> QGVNDNEEGFFSARGHRPLDKKREEAPSLRPAPPPISGGGYRARPAKAAATQKKVERKAPDAGGCLHADPDLGVLCPTGCQLQEALLQQERPIRNSVDELNNNVEAVSQTSSSSFQYMYLLKDLWQKRQKQVKDNENVVNEYSSELEKHQLYIDETVNSNIPTNLRVLRSILENLRSKIQKLESDVSAQMEYCRTPCTVSCNIPVVSGKECEEIIRKGGETSEMYLIQPDSSVKPYRVYCDMNTENGGWTVIQNRQDGSVDFGRKWDPYKQGFGNVATNTDGKNYCGLPGEYWLGNDKISQLTRMGPTELLIEMEDWKGDKVKAHYGGFTVQNE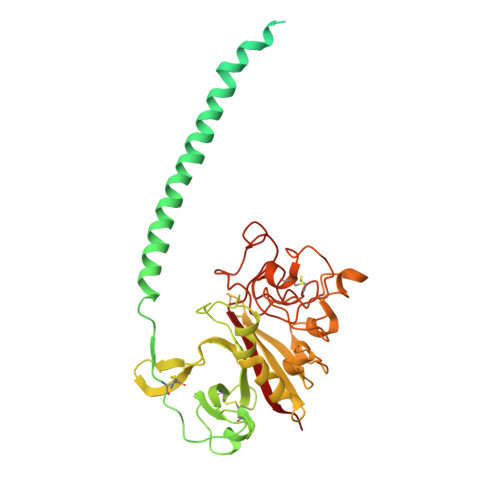ANKYQISVNKYRGTAGNALMDGASQLMGENRTMTIHNGMFFSTYDRDNDGWLTSDPRKQCSKEDGGGWWYNRCHAANPNGRYYWGGQYTWDMAKHGTDDGVVWMNWKGSWYSMRKMSMKIRPFF>AHMTRFLEEEELRSHHILERLDAHIEELKRESEKTVRQFTALKGGGSEGALEELRGQYIKAVKKI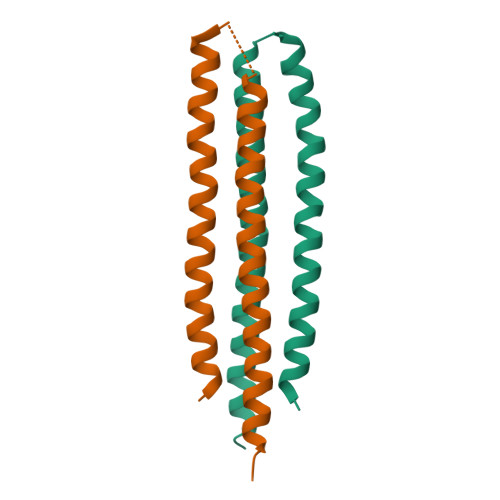KCDMLRYIQESKERAAEMVKAEVLRERQE[4x]> MEDTPLVISKQKTEVVCGVPTQVVCTAFSSHILVVVTQFGKMGTLVSLE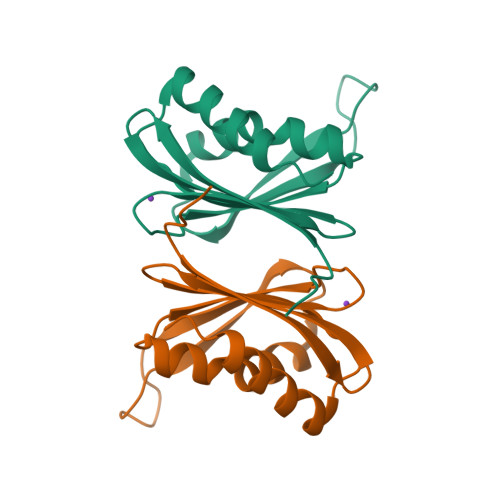PSSVASDVSKPVLTTKVLLGQDEPLIHVFAKNLVAFVSQEAGNRAVLLAVAVKDKSMEGLKALREVIRVCQVW>MNKLTIIVTYYNAEEYITGCLESIKQQRTQDFNLIIVNDGSTDQSKKLMDEAIKDYDKNIRFIDLDENSGHAHARNIALEEVETPYFMFLDADDELASYAITFYLEKFNNTDGLIAPIHSFTTQRPQFVDLDRVRVEYFNAKENINSFLRKQSACNIIFRTAIVRAHHIRFNENLNTYVDWSFVLEYMKYVNKFVRIFNFPFYFRGEVYDPFETLTLSEQNFDILFKDYVNSFYDAIKRATNPKVREFIVTKMGNKIANEFEPTRYDINERYQTHKDTLVELSKFLHVHLVKNQKLINKIETILLMNNETDKAFKVNQFRKTLRHVKNIVLRRKNKERSLYDLTDKEDNVKPKTIVFESFGGKNYSDSPKYIYEYMQKYYPNYRYIWSFKNPDKNVVPGSAEKVKRNSAEYYQAYSEASHWVSNARTPLYLNKKENQTYIQTWHGTPLKRLANDMKVVRMPGTTTPKYKRNFNRETSRWDYLISPNRYSTEIFRSAFWMDEERILEIGYPRNDVLVNRANDQEYLDEIRTHLNLPSDKKVIMYAPTWRDDEFVSKGKYLFELKIDLDNLYKELGDDYVILLRMHYLISNALDLSGYENFAIDVSNYNDVSELFLISDCLITDYSSVMFDYGILKRPQFFFAYDIDKYD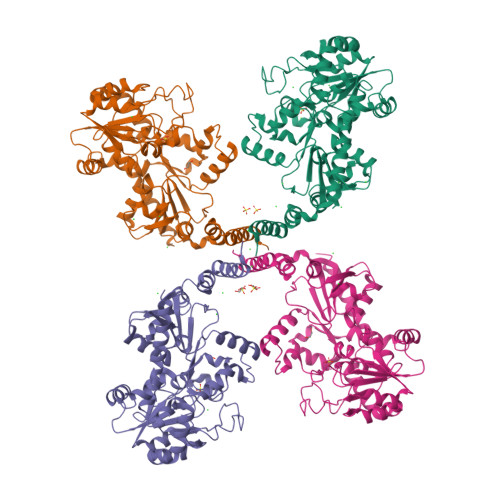KGLRGFYMNYMEDLPGPIYTEPYGLAKELKNLDKVQQQYQEKIDAFYDRFCSVDNGKASQYIGDLIHKDIKEQLEHHHHHH[4x]> MIKVLFFAQVRELVGTDATEVAADFPTVEALRQHMAAQSDRWALALEDGKLLAAVNQTLVSFDHPLTDGDEVAFFPPVTGG;> MAETKIVVGPQPFSVGEEYPWLAERDEDGAVVTFTGKVRNHNLGDSVNALTLEHYPGMTEKALAEIVDEARNRWPLGRVTVIHRIGELWPGDEIVFVGVTSAHRSSAFEAGQFIMDYLKT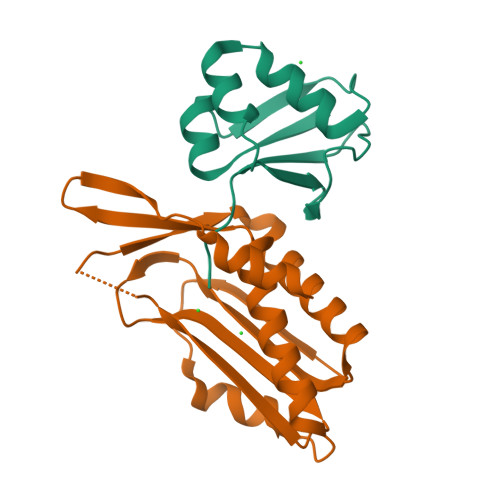RAPFWKREATPEGDRWVEARESDQQAAKRW> GAGEVKKATAEEVHARIEFLWQREQEKKKEQVV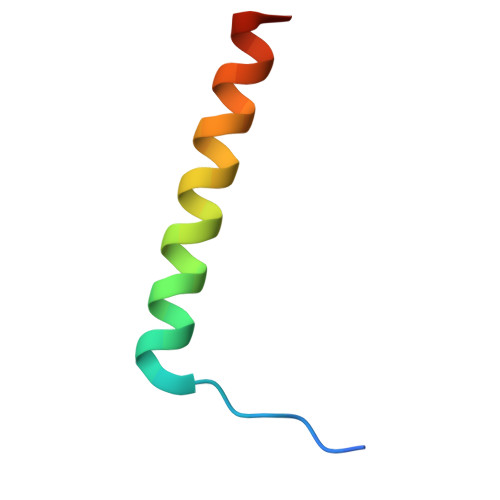SLK7-oxo-7H-benzimidazo[2,1-a]benz[de]isoquinoline-3-carboxylic 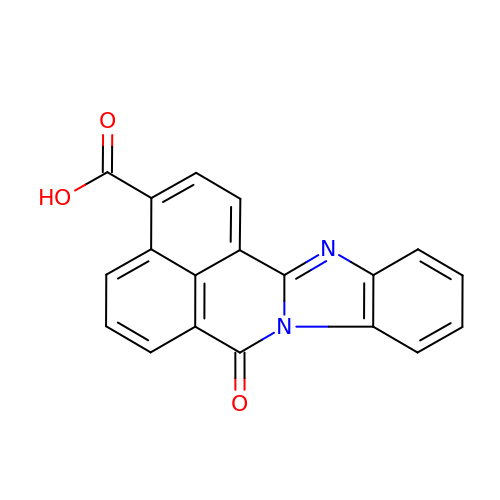acid | C19 H10 N2 O3 | MYKOWOGZBMOVBJ-UHFFFAOYSA-N>RELTVGINGFGRIGRLVLRACMEKGVKVVAVNDPFIDPEYMVYMFKYDSTHGRYKGSVEFRNGQLVVDNHEISVYQCKEPKQIPWRAVGSPYVVESTGVYLSIQAASDHISAGAQRVVISAPSPDAPMFVMGVNENDYNPGSMNIVSNASCTTNCLAPLAKVIHERFGIVEGLMTTVHSYTATQKT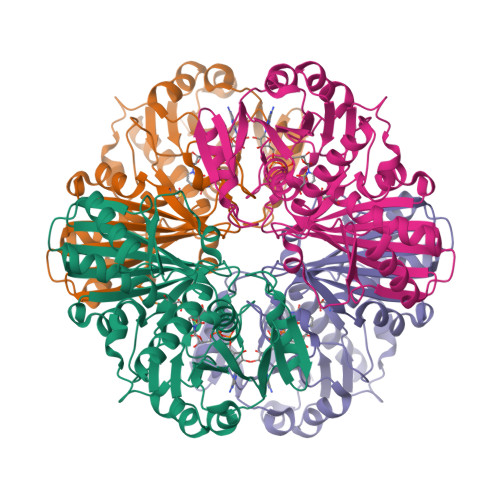VDGPSRKAWRDGRGAHQNIIPASTGAAKAVTKVIPELKGKLTGMAFRVPTPDVSVVDLTCRLAQPAPYSAIKEAVKAAAKGPMAGILAYTEDEVVSTDFLGDTHSSIFDAKAGIALNDNFVKLISWYDNEYGYSHRVVDLLRYMFSRDK[2x]> GCGCCUGGACUUAAAGCCAUUGCACU;> CCGGCUUUAAGUUGACGAGAGCAGGGUUUAUCGAGACAUCGGCGGGUGCC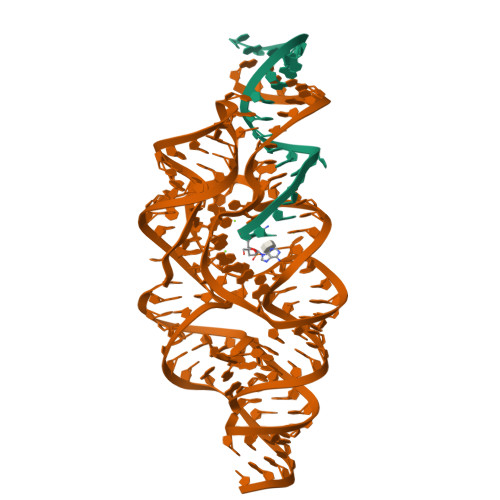CUGCGGUCUUCCUGCGACCGUUAGAGGACUGGUAAAACCACAGGCGACUGUGGCAUAGAGCAGUCCGGGCAGGAA Thousands of outer-arm dyneins (OADs) are arrayed in the axoneme to drive a rhythmic ciliary beat. Each OAD is divided into two regions, a head that contains AAA+ rings (rings) for ATP hydrolysis and a tail that holds together the whole complex. The tail is permanently attached to the MTD A-tubule, while the head region of each HC contains a microtubule-binding domain (MTBD), which binds and releases the MTD B-tubule depending on the nucleotide states. We reconstituted the purified OADs onto MTDs to mimic native arrays and determined the structures, by cryo-EM, of free OAD and OAD arrays bound to MTDs (OAD-MTD) in two different microtubule-binding states.

To further understand why microtubule binding is critical for the TTH interactions, we performed cryo-EM on free OADs. In the absence of MTD, most free OADs are too flexible to support a stable interaction between OADs. However, there exists a notable preparallel conformation, in which the motor domains are stacked next to each other. We obtained a free OAD structure in that state at resolutions of 5–12 Å for different regions. This transiently adopted preparallel conformation is different from the fully parallel structure of arrayed OAD. Upon MTD binding, free OADs are induced to adopt a stable parallel conformation, primed for array formation.

> MLSSKYSKRIAWMKTTICDSLQLKDMIVEESFQYEKNKNLLEQFLSGEGLNKIFAYYQVQEQAQNDDIKDTGAQDPVLFFTTGDLEKIQDKAVWFLRITNPADDKKKASQQDGNDNDIIFGEITPNTVPMLNALMESVYSRQIDHIITEKIQFWGVAEEEQVLEFQQHSNKFSSEVREAINLMSPGTEHFKLDYEAISGLSESEKMQHYEMKFNEWINLISSQLNDDSEVRKDEKDAGPATELIYWRSRMQKITNWSEQLKSKDFQIVKASLQRHKNHDNQRPRGDESLSKLMMEYNRLDLLLTDKLNEAKDNVKYLTTLEKFIEPLYNGTPQQIIDTLPALMNAIKMIHTIARFYNTTDKMTGLFIKITNQMIKNCKDRILNKKDNGDNPSLYKMIWEQDPAELIEVLGSCIKLYCEYKKCYNDTKEKVADMPKGKTFDFSDAQIFGKFDTFVRRLQKLIEIFSNIQQFNALAKHNLEGMDVLTNKFKKIIDDFKKKGHNLLDTANNKFDRDWVEFNVEISHLDGELQNFIDNNFNRFRNIEYSLKLLHKFQSTIKRDSLKHNLTSRYNAILHNYATELDTIQRVFQDQKSNPPLVRNMPPEAGKIIWARHLFQKITGPINIFPENVINSTEIRRYYGSYNTLGKQLTIYEMWFYQDWVNKIEQSKAALQATLIVRHDENKKLYVNFDLEIMQLIREAKCLDRQGIEIPESARIILLQEDKFKTYYNELLYALKEYERINSKIKPICKNLLLPHIEDLDLKLRPGMVTLTWTSMNIESYLYYVHQGLKKLEQLIINVNDIIENRIENNLKTVSKVVLVHLPQDTKPLSLDSFVQLQEEYINSKTDFLTSKNVEVERAVDDLLQTIMLYPLDPHVDPVLPEETKRIKRYYFWYFYQALLNSTQNSLNAMKYRVCGKKIPGANTLQNLKPFFQVEVQLNGDKVTLNPSLQEIQKSINRAATAVLRCSKHLYNWDQQNKDSTDKATFYDMIACDKEIVKVILLLTGSIQGTKNKVNEFLSGFTKFEWLCKESIQESIKKFSKNGPTLQNYEDQLKKFSQIEEEIEKIVPTYKIGAMELMTHNICTSLSTWAKEWKLQYSQDLHKRARQLLDSLTEQTKMLSTKLSKPVKDIDSLGYVMETLEQIRKEQAEIDMKFNPVQEMYSLLDNYLPGGITDKDEMDARSLLRRNWDILIQQAEIKGKEYQHKQAIYLKELKQSIKDFTNQVSIFRRDYEKNGPMVEGISPAEAMERLRRFEDEYDVKYQMYKINARGENLFGLQNQKYPELEKTDAEIKNLNKLYNLYDSVIKNIQQFKEKSWQDVSKDDLAKMEEDAGKYGEQCSRLPKDLKEWQAYRDLKNYIDSLREQLPLIISLKKPSIMPRHWEKIKEITNTKLNYENPDQFYIEEIMGAKLLDFREDIEDITESADKQLKIRTGLDEINLYWNDMQFQFGIWGKRDVPCMLNGLIVGTILERLEEDQLQLSTFNSQRHVTPFKAEVENLIRTFSDVNDTLDMWVKVQKLWTSLEPVFTGGDIARQMPLQAKQFQGIDKNWMKIMEKAVETKKVIPCCQNDMLKDFLPDLNRKLEDCQKMLEAYLEGKRKKFPRFYFVSNPTLLKILSQGSEPTSIQEDFEKLFDAITKVTFESAKDKKNPALKQITQIQQVIGRNEENISLTGYYVKCEGNIEDWLKKLEQNMQQTLKDIASAAAQQVFQVGLKEFVSSQASQIALLGLQILWTSKVNEGLERLSRNERNAMDIKRNEIKEHMNILSSMCLEDLNGAVERTKVETLVTIQVHQKDISMDLKCKDVNDFEWQKQTRIAWKTDIDECIISITDWDSPYSYEFLGAKERLCITPLTDRCYITLAQAMSMYYGGAPAGPAGTGKTETVKDLGRTLGVFVVVTNCSDQHRYRDMAKIFKGLVQSGLWGCFDEFNRIDLEVLSVVAMQVESITTARKQHMKKFMFPEEEIEIELIPTVSYFITMNPGYAGRQELPENLKVLFRGVSMMVPDREIIIKVKLASVGYLQIDLLAKKFNVLYRLCEEQLSKQRHYDFGLRNILSVLRTAGNTKRQEIKSDEEMLLMRSLRDMNLSKLVADDIPLFNGLLADIFPKLKEVPKKLYPDVEKKIPEEINAESYLINTPSFQLKIIQLYETCLVRHGFMLVGPTGSGKSTIMKILTEVLTKLGSPHKIVIMNPKAITAEQMYGVKSEISDDWIPGVFSTIWAKSNNRALKHTTWITCDGPVDAIWIENLNTVLDDNKILTLANGERIAMTENCKVVFEVENLNNASPATVSRCGQVYVSPTDLGYEAVIEGWIRNRKASGRAEESDKLGNILRKYLINMRFIELQSKECKEPMMDTSPVISVINILNLLTGCLQYFVQTQRTLSEQEYEKFIVYSMAWAIGGIYEAQDRVRFHELLLAKNAPIPQKGKENETVFDYYVSQDYLDWKICSPEEWVPPQSLQFSQLLLPTLDSFRAEMLLNFILTQPKSHTCSNSALLIGGSGTAKTSSVLLYCNKFDPQKMLFKRTNFSSATSPFMFQSTIEAECDFKVGKEFAPPGNKMMTIFIDDMSMPFVNKWGDQITLELVRQLIETGGFYMLDKTQRGNQRKMKNLQYIGAMNHPGGGRNDIPNRLKRQFFIFNMILPLSIEGIYGPIIKHMFKQKYFSDSTYKVIESLTSATIALWNKVKSTMLPTPAKFHYVFNMRELSRIFKGILTCKKDTINDAPKSMKIKPELFLVGLWRHEAERVLADKLVNNKDKDTVMGYIQEVSLESFSQIENEILEKYSSEKTFLFCDFLRPDVINEDGIIEEEAPKIYEAIDSLTELRKRCNFLLSFYNDRNPSKKMPLVLFDDALKHLLRISRIIRQPRSSGLLVGVGGSGKQSLTRLAGFIGKNLIQQIIVTKTYSDKDLKEDIKKGFDDAGHLGKQVTFLMTDSEVKKEEFLEYINMVLSTGEIPNLLAKDEREVWLGDISQAYCKEKNLGNIDPPQSELWTYFVDRVRDNFHIMLCFSPVGQKFRERARKFPALFNECTIDWFLPWPEEALVSVAETFIKNFDKLDTKEETKQELMKHMGNVHLMVNEICDEYYQKMRRQVYVTPKSFLSYLNSYKTLYIEKYDELDQQEESFKIGLNKIQEATITINQMEISLKEEEIQLNEATEKTNQLLANLDKESKKANQKGEEVAATNKQCEIQAEQISKEKEEAERELEAALPALRRAQEAVDSIESKDIVELKANKKPLDIIKYIMDAVLVFFKARLIPIQIEERVFNKKEGKAVLFLKESYDESGIQTLGDMNFMKKLKEFEKDSINEETIELLEPYLNQSEDWFNDTFATKASKAAAGILKWAFAIYEYHQKSKIVKPKRIQVAIAEGRQAIALKELEKAREDLAQIQAYIKNLKDVYTKQMEEKNELEMKAAKTKKKINTARTLITSLSGEKDRWGKGAQDISDQKRKLVGNVSLSTAFISYCGPFNAEYRNKLAQQRFVVDMKKRGVPVTPGLELTSFLIDDATIGEWNLQGLPKDDLSIQNGIMVTNSARYPLFIDPQGQGQNWIRNKLSASIIPERCITTLSHPKFKDMFLKYCMESGLTLIVENIENEVDPMMDPVLERQIIVKGKTQFVNVAGTEMELSKEFKLFMTCRLANPSFSPELSAKTTIIDFTVTQSGLEQQLLGKVISKEQKALEDSLNQLLADVNQNQKDLQRLDKNLLERLINSQGNLLDDTELMDVLNNTKTQAKEVAAKLIDAEIKTKEINEKREQYRPVAIRGSAIYFTMIEVSLVNWMYNSSLEQFLKLFIESIDLSEKAQLPSNRVKNIISFLTFHVYRYVNRGLFEKDKITFILMMAFKILTTAGTISSGDVSLFLKSGDALDIKSERQKQISYLEDNQWLNILALSKHTFSGQTLPFFKELPDLISRSENQWRNWIDKNDPENFPIPDFAESINQEKEIGSFISLCLVRSLRNDRTLIATQNFISNVLGKEFTDPISYPIEGIWQESSNMDPVLFLLSAGADPTSSIDELAKKKKKFPCEKVSMGEGQERVARQVIMKGFVEGGWVILQNCHLGLKFMEEIETLVSPINQIHEDFRLWITCEQHPKFPLGLLQKTLKVTNEPPKGLKAGLYKTFTTIITQEFIDKVDHSNWRSLIFTICFLHSIVIERKKFGPLGWCVPYEYNYSDLEASLLYIEKYLTNLMSTPQPNSHNLPISMNVVRYMICEVQYGGRITDDLDRELFITYGETYLKDGIFGNDYFFYDIMVDGSGQKFKYRIPQNPSAELIKYQEYIAKVPTVDNPEVFGLHSNADLTFRLKESKEMINTVMETRPKDSSVGGGKTREEIVQDKAKDMLKNLPPDYNDVEVRELVSKLGGPNPKTSTERGMTVPLNIFLYQEVTRMQRVIGLVRKTLQDTILAIDGQIIMTPEILEAINAIYDAKVPNSWLYDPSGAEISWLLPNLGSWSTSLSDRNKQLNDWLRSGQRPILFWLTGFFNPQGFLTGMKQEVTRNHKKKDGKGGEAWSLDDVVYSTTVKEREKEKDIEQPPAEGVYIKGLYLEGCKWSKNGLDDSDPKKIFADLPILHVSAINKKKTNEQDRMSNTYLCPVYKYPKRTDKYLIFRVGLPCEGSNNPSHWKLRGVALLCSTE;> MGDHSQKDSPEDFIINRLSQALGIQKEKIKKSLETQQDDKGEVTNKDEFQGFIQQDNSTNILWVSGQSEKCTFYYGQLPPIDKFKKKGIAVIKLGLHKLTNENVAKDVVVVEITNNLLEHLNSVFNEIMSPVMQNPLNQQGWTDLVAKDLMEKFNNYVAQVYVLLGQIKGKTMLPLPSHKLTSSDTTPDKDKAHVFEGSIITWTKQIKNVLKLEPEQLLKYGNDPGPLAEIEFWQNKRDNLNLIDSQLKSVEVQNILHFLDNNKSTYTTPFTKLQAEVKKARLEANENYRYLFTLKDLFSKLQESQPSDFPTLYELFIPIMHTILLIYNKSKTYNQPPRLVVLIREICNAIISNAQAFVDKDTIFSLIDSKETTEACDKLQVTLDVCSKFKDAYFEYKAKAGGNWKLTSNALFVRLDSFLERCQDILHLTNTIVQFNKLEKIELGGTKGKTLTESIAQIFKEFEEAVQAFTSVSYDIMNIAEKKFDDDFYEFRSKIKELERRLASVITQGFDDYDTIYGRFKLLDNFEGLLTRPIIADELEKKHIVLLEMYKQDLKQVQSIFLEGKQFVDSMHENAPLFLNMPPIAGALTWCKSLRDRIQEPIEKLAQLGQGITEREEYKDVQKLYTSITKSIKDYEDQKILSWEKEVEDSSQDKLKQTLLCKDENDLIKVNFDPSLVRLLKEVKYFLLLRLEVPTTAKDIYTKAETYRTQIVALDMIVDNYNHIKTCLLPVEEPLVKKKIQDMEEEVKPGIEEIRWKSTNIDQFISKSKSIVDQLFETVNKMKDSLQKIHKSLANFNVKIIERKNRPMSPDDYDQFLKAIFSNKLTIVKDNGNQIQKLVKEVLDAVKADKKQNSWKNYNDYVNVIVIEGISTAIQTALLHLNEQINPVFIKRNDISPLFDIRLELGQSGIQFDPEIGESSNQLTVRNTIRNWINDFFNIAGTIQRLDTTMPGDFLQEIRSFFEIKQCLAMITQNLEWIENECNQFRARFDTYSYLWTEDEQISFNRFLDENEPKDEDGKGGDDDEGENTEKQNPLLKGCRAKIPNLDLFDEKITHLKAIQQEISRIKTPEDISWLRINLQPMKTALDARVTRWIRVYTDFLVNQFRTTQKNLLDFIEKTKDGIKKNPADHENLHDKKLLMSVMKVISDVKDVEPRREGIITRMKEMVTKLKKHNVPITEKGTDDPLQQIDNANSNFIEIYGRVFKVKADIIPLQAEETQNIKRDLDIFMKEVESFRKEFMQKLPFDYTESMGYENINNAYDTIMVYYHKLTAIEGRALEYNNLEKLFELQKSNYKQLKDCMNDLKNLKTMWDAIALIHFQYNDWKTKPWRQIKADILLDTNKTLGTQIKNLPKEIRNFKGYNVIVEKVKNMGTVLPLVSALHSEFMEDRHWSQLKQITGTVFDHNSLSFYFEDILALNLYKYENTVNEIVDVAQKEAKIEKKLKNIEQWWSKQVFEFTEYKETKTFASLDNMMEVLDQHSLDLMGMKSQGKYVEFFYDRVEDWREKLGRVDVVVNEWLKVQKNWKILYNIFLLSEDIRMQLPEDTKVFEGVDKEFKDMMSEVSANPSVVEACTIERRDVLVGWSQAIKKCEKALNDYLEQKKKSFPRFYFLSNQSLLTILSNGQNAPKVCEYLGDCFDGLKTLTFEPPANPAETSKVGIGMISKDDEKVPFSSKFICEGAVEHWLLNLEFRMRETLQEILEGAKNTADLWDSGDKPREEWVEGYNAQIALLTTTIVWTEDVGRAFEDLAGGSETAMKECQKLIEVRLENLIKKVRGDLHILERWKIINIITIDVHSRDVVEKFVIQKVSEAESFAWLSQLKFYWENKPDSDMHLRQTLRFPWEKDKNKNKCIIRIVDWFRFYSYEYIGNAIRLVITPLTDRCYITLTQALNLTMGGAPAGPAGTGKTETTKDLGRAIGIPVMVFNCSDQMNKDSMAQIFMGLSQSGAWGCFDEFNRISIEVLSVVSTQVKCVLDALKEKKTKFSFVEEGEIQLQDTVGFFITMNPGYAGRTELPENLKALFRSCAMVVPDLALICENMLMSEGFTMARVLSRKFVSLYMLSRELLSKQKHYDWGLRAVKSVLRQAGKLKRGDPDMPEDPLLMRALRDFNMPKIVTDDKVIFRRLIGDLFPKLDPPTKQNPELKKIVQDTTKKDMGLVAEELFVTKVVQLAEILEVRHCCFVIGPPGSGKTCVWKTLIKSYINSGEDAEYDTLNPKAVTSDELFGAYTKTKEWKNGVIAVIMKNQVKNEEKYKATHMHKWSVLDGDIDPEWIESLNTVMDDNKVLTLVSNDRIFLTPQMRLIFEISNLRNATPATVSRAGVLFINETDIGWMPYMNSWLERSQINILKQQKEMANMPEYPVIDDVAKSVFYRCFQSYFEQNIDVHDKNRVRHICPMVDIAMIQTICTILDALLIQHLPKLKQMKEEDEKQALEAFFIFAGLWAIGGPVGGGQDDSKDMKEFNTVWKGAAKVKFPEQGLCYDYYYDINENKWNTWKVEDYLPNDQPLFSKIYVATIHTTRLRYMIDIHLQRRKPILFIGSAGTGKTAVVRDYLNSTRPEQVSHKTINFSSFTDSLALQKNIESMVEKKNGRNYGSATNKVLICFIDDFNMPYVDKYGTQSPIQLLRLILDYGSIFNREQLEERKFLQDLLFFGCLNQKSGSFTVDLRLQRNFSVFSMYTPSSDVIKTIFGSILNAHLSTIDDKAQKMAFKLVEATYFTFDKILKNTTAFAPSAKRFHYQFNFRELARVCEGICRTTPGQYSGGDQGKLVRLWAHEMKRTFEDRFIANEHVEFFRRYLTEAISKCIGEFPETENPIAEPLIFTGFVAAHQGLDQQYTQCTIPVLKRVLDDKLEEYNEVKAQMNLVLFQQAMEHVSRICRILDMPGNNALLVGVGGSGKQSLCRLSTFINGFEIDQLVVTASFTINDLRNNLQEIYKKIAKPNSIARVFMITDSQIKEEQFLIPINDMLNSGWIFDLFPKEDMDSLVSGVRNEAKGEGVDVNNLTALTSYFLDKIRKNLKVVLCFSPVGDTMRIRSRKFPGIINNTSIDWFHPWPHEALIDVAFRFLEEIEFPTEEIRQSISLNMAKVHSSIDTANEKFLKLERRYNYTTPKSFLELIDFYKKLLTEKRETIQRQIQRYEMGLNILAETQNKVQGLQEELKVKMVEVNKQREETDILIEKVGKESALAEEEQTIANAEEEKTNVAAAEAEKISKEATEALAEALPALRSAEAAVDCLKKPHVTEMKNLGSPPAGVIVTARVVLILFNQGITLNDPDEKVWKKAVTFMNNPQAFIDKVKSFDGENIEPNIIEQSNKIIQDPSKKFNEKDMAGQSYAASKLCAWAVNIVTFNKIFKQVKPLQDAQKQANEILEEKKKELAIVKQRVAELNARVNSLKRQLEEAEARKMIVEQDAARCQSRLSAAENLVNGLAGENKRWTQNVKFLKENIKSMIGDSLLASAFVSYIGAFSAKLRLELWKNTWLPDIIEKGIPITEGIEPLKILTTEAIKSKWKNEGLPADPMSLENAAIITACARWPLIIDPQLQGSTWIRGKQGENLTTISLSQPKWLGALTSSISSGRAVLIEGIQQEIDATLDPLLQRAVKKNGNQLQLEIGGDPIDYDPNFKLFLMTKLINPHFRPEIAAQCTIINFIVTESGLEEQFIAMVVNIEKNELEMAKQDLVKKQNEYAVTLDKLESDLLQSLSEADPATILDNTELIQNLDKTKKTTIEITEQQQKAKVTEAEINIQREHYRVVAAEGSMLYFLVISLSVMDHMYQYSLESFITFFFKAINRTTVRDENRIPTLILNIRQTIYQWISRGLFEKHKLIFLTLIVFRLMQKKIIDVAYEVAEMDFLIKCPARPGVENTLDWLPNISWDQIQGLINLEEFRNFAHQLEKEAPNRFKDWYNELQPEDQKLPLDWKRLDSMPFKKLLVLRCLRPDRMTISLNNFIRAVLPQGDAFVEMDQKLAFSEILESVINEDSESTIPIFFILSPGSDPVKEVEKIAKKKRIEPGKNFFNIALGQGQDEIARRRIEEGNKEGHWVMLQNIHLMPTWLIELEKILDSYSGEAGGGNSEFRLFLSAEPSTGIPIGILDRSIKLTNEPPAGLKANMKRAWTYFSKEEIEDKDPKIKSILFALCFFHSTLIERRRFGPKGWNMSYPFNMGDLRDSYLVMNRYMEQNQGGKVPFNDLIYIFGEIMYGGHIVDDWDRRLCNSYLFNTMHEQLFDELELFPYIEGKGLSFKVPGQNPYEKYIEHIETSLKQETPLAYGLHPNAEIGFRTDQCKTLFNTLLELMPKEQSRDEKSSDIKSSNEMASDLIKQLLEDSELKNKIFNMEEIKNKIDAENKGPYQNVFLQEIEYMNALLSEIVKDLEEIGQGLSGLLTVSENMEMIIESIALSRVPASWQKLAYPSKRGLQSWLANLFQRIEQLNIFRDDPYSIPRVVMISRFFNPQSFLTAIMQVISRAKAYELNKLYIQTEITKRSIEEIEGAAKEGAYVYGFILEGARWDYQLGQLEESKPKEMFSVLPVTYCKAIPLPPEGKEDKSLYQCPVYKTEDRGNTYVFTAQLKTRFPPRKWILAGVAIIMDVEGVSDEVKKDKK;> MPQPLVWTQLKQTGTTQPTARSGHTIITVGKTHIMFGGLDNDKNNYKDGKIAPNNQVFTLKLTQNNCEWRQIACQGDVPLPRCYHASCAISADKMLVFGGSYTSNLRFNDTYILKTTSYQWSKPANQISGGEPKNAESKIGAPQPRYGHSATFFEGKVYIFGGHGGINYQRLAFNDLYVLETENFEWTRLEPKGNPPDPRGGHSAAMMANKPQLMIFGGWSFTSQYSNIMIYDIEKDEWVDPEIAHEIPKWNLSGIMAPSIPSWKYFIFGGSVGSFEEGGNRTNSRFVDDSFVLDIDTLSWSSINLEADETSKAVCKPRPRESASIFYDSGESRAIVFGGWANNWLNDLWALNVSTITGPPYAIFSIKPALGPLTGKTKVLIEGDGFKDTQNISVKFSGGKLEKEVNGTFVNEKEISCETPTFDYPRSVEVTVCMNKGDYTITKSAFTYYLNTKADKTIAYGPGLLTENLIGVQTTIVIQARNKNDQNRESGSDEFVVTIRNPAKIKKEEEVKEGDKANTKNTIKEDEEEEGEDEEENKKKKEAEKAAAEKAAAEKAAEEEQGEAVDPSLVPFNIVDNDDGSYFIQFTSEEEAVLEIDIKFKDENNELHSIRGNPFRCGFVKGSKPNNNDLTGSAVMNYISKQLKDIQEFIENTKENIEIRNKNIRENVSELINVMINLEKVRVKNDDDVLTLDTVEEMLNFLKKKDFGKDSDIKKCKKLQEEWKNLAKMAQAVKKDIQNPVKTESDKTKENIKKFEEITLKEYANSLKKESFFIYKTGVSESFKRIGEVKQKVDEFEVQLNQYEDFARMFEFPDAVIGSKKLMEQIRTDVSSVEKLWVRIEISEKTMDEYKKMKWGSINSMDMEDEIKKLRKALTDLRGIDKRSNAFIGITEELKKWATFLPLLGELKDPSMNSEDGRHWKKLKDLVKKEFDVSQELMLEIIWDLKLFDYKDGIEEITDQAKQELKMEKALKKIIDFWRDIEFELVQHKNTDIHTLKMSEENFETLEDHQLQINNMLLSKYVAYFEKEVEKWKYDLGSVYDVVQLLLEVQKTWSFLENLFIQSEEVKRELPNESAQFVGIDKDMKEIMQKGCDIKNCLKFCTIEGMLKRLENIQAQLKVCEKALNEFLDSKRRAFPRFYFVSVNDLLDILSNGNSPAKINRHMSKIFQAIDNLQLKEDSSGGRPTALKMISCVGTEEVDFSSPRLLQGKVESYLKDVIDTMIGTLKSVANSSFKNFQSMTRKEWLKSDPSQITLLVNNIIWSKAVEDCFLKLQSGDINAMKLFLDESIKQLTELIGMVQGDLSKPLRQKIMCLITIDTHSRDVVHRLINEHVRKAEEFQWQSQLKFYWVDNDAKIKIADARFVYNYEYLGNGPRLVITPLTDRIYVTATQALHLKMGCAPAGPAGTGKTETTKDLANALAKACYVFNCSSEMNYESMGNIYKGLASSGCWGCFDEFNRLLPEVLSVCSVQFKAVTDAIKQNVERFIIEGDEISLDPTCGVFITMNPGYLGRAELPEGLKALFRPITVVVPDLELICENMLMAEGFIEAKILAKKFVTLYMLCRDLLSKQLHYDWGLRAIKSVLVVAGGFKRSEPEIAEQALLMRALRDFNIPKIAFQDLYVFHGLLGDLFPGINIKPKKDLDFEKIITDVCIENKLDPDPEFVLKVVQLSELLAIRHCVFVMGPPGAGKSTTWKILAKAQDKTNKKTTLIDIDPKVVSTKDFYGYNLPSKEWKDGLFSKMLRSLAEQPDTNPKWICLDGDLDANWIESMNSVMDDNKILTLANNERIPLKPHMRALFEIRDLRFATPATVSRAGILYISDEVGYQWRSYVKSWIKQEFSQDQEMSKNLDTLFGKYVPDTLDHIKKHCRFLVPVSPISQVISICKSLQTLLKGDVKNLEYLFVYALIWAIGGALAEKDSIDYRKDFSTWWKGAWKTAVKFPSKGTIFDYYVDQSGDSSKFVEWSKRLENKEFDPQVETMGNITVNTIETLATTEFIKSYLMVKHPSLLIGNSGCGKTQLAKGILKEIVQAKPENYAYQLINFNYYTDSTYLQGQIEQTLEKKAGRQYGPPGKVQLIYFIDDLNMPQLDAYDTQTAIALLRQLADYGHFYDVSKLALKDIINTQVLAAMNPSAGSFFVNPRYQRHFWTISIPFPDNESLSLIYITFLNGHLKRFKSTIQEYSNIIVRASLMLHQAVTQNFRKTAINFHYEFNLRHMSNVFQGLLLSDPNKFTEPDKLIKLWIHECERTYGDRLVSTDNLKTYKENIFDIVKKSFSKFNFSRYFGNNPENLIYCNFIAGINSDRFYDQMPNNEMEKHISEALKEYNDNNAFMGLVLFEDAMKHVCRICRIVLPSSGHALLVGVGGSGKQSLSKLASFIMGYTTFSITISATYSMVDLRNDLQQLYFKCGPKEEGILFLFTEGQITNERFLVYINDLLSSGEIAELYTLDEKEAMINQVRAKVKGEGKPDTRENCWNWFIDQVKKNLHMAICFSPVGDMRRRARQFPALVNCTVIDWFQPWPYEALFNVAKSFLEPVDLGDDKVREAVVKFMPFSFTLVNDLGLKLLEQERRYAYTTPKSFLELISLFTNMLAQKRESLERNKERYETGLVKLKETAEQVAIIEVEVKEKQVEAEAKKKEADAFAEVVGREKDKVEKENSKATIEADKCGLIKQNVEAQKSSTQQDLDAAQPLVEQAKSALNSISKKDFQQAKSFASPPAGVPEVFAATIYLLAGYFNEAIEIDKNKKPKDVSWKSSLKLMKSPEEFMEKLLNFKDVVDANQVPAANVNIVKNQYLNMPSFTPEQMASKSAAAKGICSWVVNIVKYYDVIQDVEPKRKALKEATEQLEEATVKLNEVEEVVRKLNEELNKLKAENDKAIAERNAAISEAERCARRLNLAQRLVTALSSENERWGKSIIQLEDQLKLMVGDVLVASSFVSYSGPFNKKFRNIMINQNFMKFMKEHTIPMSPDPNPIKILTDESTIALWNKQKLPSDSVSIENGTILTNSARYPLMIDPQLQGITWIREKEKANNLKILRLGSKNINRDLELSIENGYSAIIENMNERIDAILMPIIARSFIKRGKNKIIKFAGKDLILHPNFKLFLHTKLSNPHYPPEIQAEAALINFTVTEAGLGDQLLSLVVARERPDLAKMKIELITQQNDFKIKLKDLEDELLYKLANAKGDILDDIELIENLEYSKKLSVEIAEKVAAAKITEAKINETSENYRPAASRGALFYFLLSDLSKVHSFYKYSLESFIVVINRAIDAISENKIYGKTTMVPYGDETYASNQHEKEEEEEEEEHQQAQQQQNQEEQQEQKDEENKGPVEEEQPEGENKGPVEEEGAEGQNEGPVEEENAENQEGEGEEEGEKQQKAKDSDEPMSPRSLKKRVDELIESLTYTAYQTTRRGLFESHKLIVAAMLCLRVLLRSEELNSDEVDHLIIGKVDVNPTPMPDALKSFLNDNIWAACKALETIHQFQGFCQSLETDVLQWKKWYSEEKAETADLPKAFKELSKFHRLLLLRALRPDRLPSALSQFVHDKMGERYIEQPPFNIFETFQETSKTVPIFFVLFPGVDPTPDVERVAATFDVSANNGRFINISMGQGQEDRAKKALFDCAQKGHWIMLQNVHLMQSWLYGLNGLEGFLESVFASPKTHPNFRVFISSEPPNVLLPLMQIIPESILQGSLKIANEAPQYLKANLRRAYNKFDQEFLDKCDKKPTEFKSCLFALCFFHSLMLGRKKFGTQGWSRVYNFNDGDLTICADVLYNYLSKYDQVPWDDLRYIFGEIMYGGHITDDWDRRTNRTYLKVLIRSELLQQNFNLAPQFKSPDPSKFDYEAYRKYIEEKLPIESPQMFGMHPNAEIGYLTQTCDQVFNTILEVQGGSSGGGASKKDDGVMVTLTDFKTRCPHDFNMLLIEEKVKEKTPYIVVCLQECERMNGLLKEIKTSLEDLRLGLTGALNMTDAMESLQQSLSFNKVPDTWEKKAYFSKKPLSSWFADLIERNIQLQEWCKELVTPTSLCISYLFNPMSYLTAIMQFTARAQGLPLDGITIQTNVTAMKGPEDVVNPAENGAYIHGLFLEGAAWEIGGQGQDGYLIEQKPKELHPKMPVINAVAVPLDKKKKNGQYDCPTYVTSARGQTFVFTANLNMESDDSDPNKWILSGTCMLMSDD;> MPPKQTKVVASRKTVMPISRAGRAQIRRKDSNTQNNMNDQGMEDEEIDQQREGMKNQYEQLTAQELNEDMPSKMLEPKNPQAPKNITVYDYYTRKFKTDELVDQMIVHFSMDGDYIWKESNEYKTQEEIRDTKKALIKEAMRKQESEEPGANHDEEAIKQTLRNKFNYNTRECQTINPSIRERGVSTEPPPSDTICGNITQWEIFDAYYAEIMKDHQIENKKKKEVDQDKKQDQSMYSTSFKRCCKIMERMVVQNDQEDKYHDYRYYWSQGDNLEAGKNEGHLLPIWRFSNEKQRKKNVTSICWNPLYPDLFAVSLGSYDFTKQRMGLICLYSLKNTTHPEYAFNCEAGVMCLDFHPKSAALLAVGLYDGTVLVYDIRNKHKKPIYQSTVRNQKHTDPVWQVKWNPDTSKNYNFYSISSDGRVMNWILMKNKLEPEEVILLRLVGKNEEESTLIGLACGLCFDFNKFEPHIFLVGTEEGKIHKCSRAYSGQYQETYNGHLLAVYKVKWNNFHPRTFISASADWTVRIWDSKYTSQIICFDLSMMVVDAVWAPYSSTVFACATMDKVQVYDLNVDKLNKLAEQKIVKQPKLTNLSFNYKDPILLVGDSHGGVTLVKLSPNLCKSGPEIKQTEDKKAMEEFKNVKIEDYEREKMENLLAVVSKWEREDA;> MAEYFTYSKKRKEFNNPINFQDTETRYGGIQNQVVNINQYVQRNPNFIDLDNIAELSEHSVNTERVKTGDRGMSHKEGGWPGNVDPNEAQETGRFKKRIEKDTSFPQAVKDLKEGVEKCIYQNNQIDLLEEYFEGETSEHVVENLSSKTLMLFKDEKEICKRSVSEISWHPEGPTKVAVSYAIMRFQQMPEKMPTQAYVWDLLNPNSPEIKLMSPSAVTNISYNQKIPDQIGGGCYNGLLAVWDGRKGENPIMISPVENSHYEPVTHFHWLMSKTGSECVTTSTDGKVMWWDTRKFEAGPVEKLNIIEGLGENEEIIGGTALEYNVEAGPSKFLIGTESGSILTANKKLKKPVEITTRYGLDQGRHLGPVYSINRSNQNPKYFLSVGDWSCKIWVEDLKTPIIRTKYHGSYLSDGCWSPTRSGAFFLVRRDGWMDVWDYYYRQNEIAFSHKVSDSPLTCIKINQTGGAYHNSGKLCAIGDQDGTVTILELCDSLYTMQPKEKDIINEMFEREYRKEKNLETIKKQQELAKRQVQKDMGSQKEKWEKKKLEMIETAEASFHENLAKNPVNEEEFNELDSPSEKRKKTNQNQGREQEEQSREEQEASGNFNQQQQQQQEEEQQQEGEQQHHQNQEHQNGQGHENGQEEGEENGEEGNQQENEGQEENEQQQE;> MAQDINADDQLKQLSALEGANGYVIFNESGIPLKRHEKSISHEKAVHIAALVSDLWNVSKKVIQRDLKTPENDIEVIRLRTKHSYEYIITQSGDFTMLAIQLCGKAIEEAKKAAAAAAAAAVVQEENKEKEKK;> MIYKTSKEIQKSDQRIIQQRVENSIINNQIYQKSLKRKTSKRKVRHQANKKNFQKEMSEVEDTLNRIKTHKTVLGYLIVNSEGGVVRGAFKDEEESKNIANSIPLLTKKARSVVRDLDPTNDLVFLRIQTKLNEIMVAPDDEFSLIVIQTKGEKRDEND;> MSHLDKVQPVIKNSDMSVEMQKEVEEVAKKAIDYCNTDKEIATFIKDDFRSRYHGTWHCIVGRNFGSFVTFERSYYIYLYVGQLAILLFKTG;> MEQEKAVTDMDINELRKLMIGKAIINSSDMQGDLLQEAQDVIQSGIENNSAPVLNIEAACKYIKENLDKKFGPTWQCIIGEGYAYDVTVQNNTLLFMFYNGNLAVLIFKS;> MASNQQQKEDPKEQQQQYKTFMGARVLWPPECADDILEGAIRETQDALKKFEIAREGQKIAEHLKKYMDDHFDPYWHVFFGKNFGCQAVHNKNRFIYFYIEKTAFLMYQTQ;> MGDHANEQIIDMPENSEMKSMKNDAFSQAKFAVENYKFENKISSHIKKFFDEKYGPNWHCVVGKHFNAYVSYDSKNFIFFYEGQLAILLYRKG;> MSDSDSDEGRVVEEPLPPHIIRFNDMAQHLLKKVIRQADVLIKENPQGLEKDIALNLVKFVKSQPEFKIGDGEWQCIIGKNFGCSLTFDANVLAFFDLLPSRKSILLFKSG;> MNHEPEVKATDMEEDMIKRVKEIAINAVKEYKQEKQIAHYIKYEFDKIDGYGWNCIVGRNFGSHIIHQTKKYIFFKINELCLLLWKA;> MGDTDKEYISEEVQKAIDDSVKQVFGIKDDSSQVTITYNKDKVNLWTQQIIDYTIRGLNKLGKHFKYCVTAILQQTNHAGISVQITAYQDTNTDGSLIQCYEINDIYAIVSVFAMAV;> MKGTYLYLNIYKRKREASLITLNYIKNRFYPSKIQKIIKELFEDRLKGVEYDPNNANQLSERLVLELREKIKRGKVPRYKIGVQVVFGEIKGQGLRIASKCLWDVQNDNYASYTYTSEKVYCTGIVFGCYFE;> MSKKQKKEITTTVTSEDHFMTFYNENNKKLIVVDVYPGWSGPCTAMYPTYNQLMISIDDFEKRIDILLLDQDKLVTYKNDKFHATCQPKFLFISEGKIIDEVLGTNIPVFIEKVNKYIPLSY;> MSKGTTCQKAIVNWEAANPGKNPSEAEEIKLIFQIPPIEKMDGPVLNTLTKCKKLSLSSNSIDKMISLNMLRNLEILSLSRNVIKKISGLEDIGGTLRQLWLSYNFIEKLDGLNNCSVLQTLYIGNNRIKNWEELDKLKDLPELENVLFYGNPIYEQVKEDPKLIVLKKLPTLKNVDGYIIDDSVLEKVKQIADIPISAKQL> METFDPTELPELLKLYYRRLFPYSQYYRWLNYGGVIKNYFQHREFSFTLKDDIYIRYQSFNNQSDLEKEMQKMNPYKIDIGAVYSHRPNQHNTVKLGAFQAQEKELVFDIDMTDYDDVRRCCSSADICPKCWTLMTMAIRIIDRALKEDFGFKHRLWVYSGRRGVHCWVCDESVRKLSSAVRSGIVEYLSLVKGGQDVKKKVHLSEKIHPFIRKSINIIKKYFEEYALVNQDIL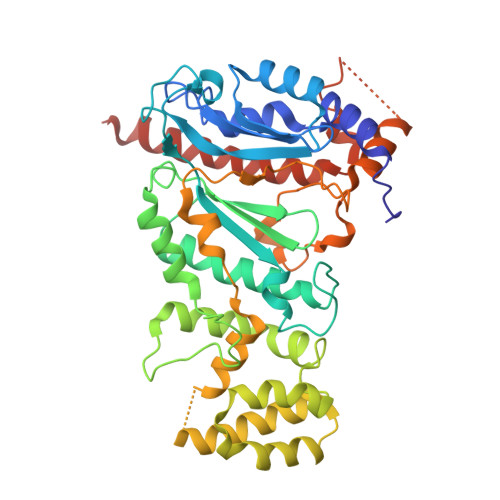ENKESWDKILALVPETIHDELQQSFQKSHNSLQRWEHLKKVASRYQNNIKNDKYGPWLEWEIMLQYCFPRLDINVSKGINHLLKSPFSVHPKTGRISVPIDLQKVDQFDPFTVPTISFICRELDAISTNEEEKEENEAESDVKHRTRDYKKTSLAPYVKVFEHFLENLDKSRKGELLKKSDLQKDF>APENPGEPGEAGQALFKADFEDGNIGNWRARGTEKLEVVSGIGHNSNRSLKTSSRSETYHGPLVEVLPYLQKGSTVHISFWAMYDEGPATQVINGSLEK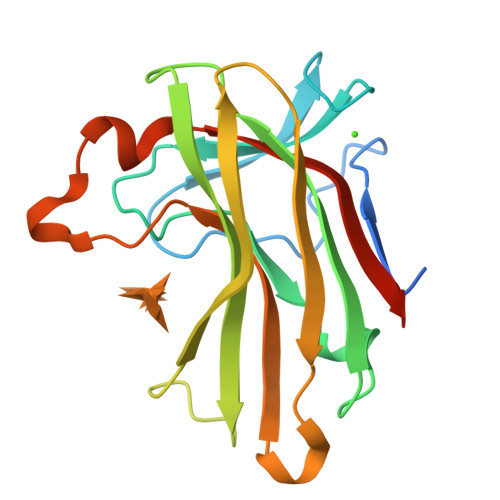EFNRDTANLEYAMFASTTLNKGQWKKIEADIIVPAESTGISGLRMYAETPWKQSSEVTETDTIPFYVDDVQITATEAIAIEK[3x]>GSPNYDKW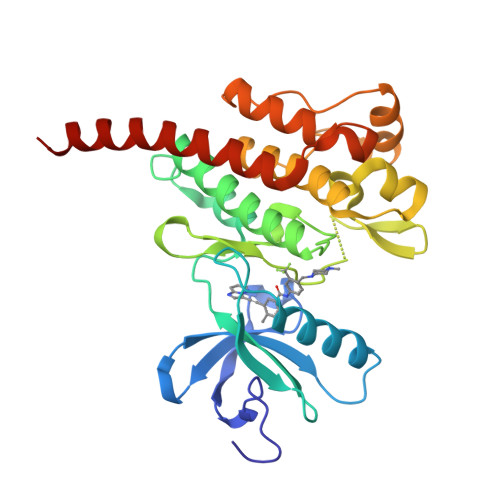EMERTDITMKHKLGGGQYGEVYEGVWKKYSLTVAVKTLKEDTMEVEEFLKEAAVMKEIKHPNLVQLLGVCTREPPFYIIIEFMTYGNLLDYLRECNRQEVSAVVLLYMATQISSAMEYLEKKNFIHRDLAARNCLVGENHLVKVADFGLSRLMTGDTYTAHAGAKFPIKWTAPESLAYNKFSIKSDVWAFGVLLWEIATYGMSPYPGIDLSQVYELLEKDYRMERPEGCPEKVYELMRACWQWNPSDRPSFAEIHQAFETMFQESSISDEVEKELGKRGT[2x]>ATMTLTDANFQQAIQGDGPVLVDFWAAWCGPCRMMAPVLEEFAEAHADKVTVAKLNVDENPETTSQFGIMSIPTLILFKGGRPVKQLIGYQPKEQLE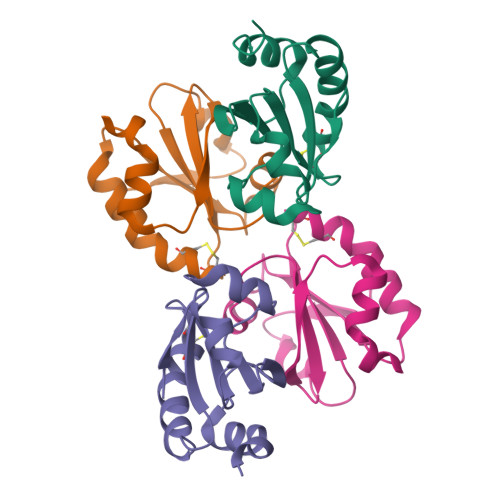AQLADVLQ[4x]>HMGIEY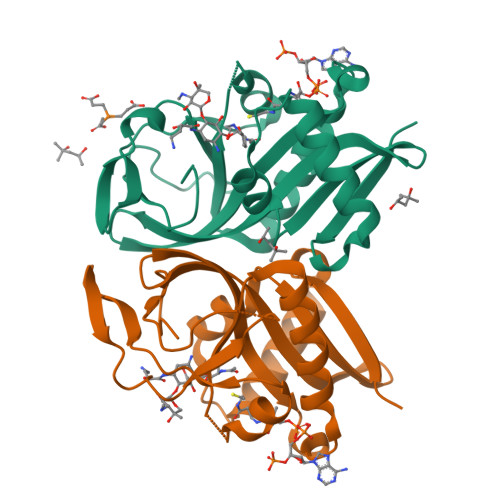RSLHTSQLTLSEKEALYDLLIEGFEGDFSHDDFAHTLGGMHVMAFDQQKLVGHVAIIQRHMALDNTPISVGYVEAMVVEQSYRRQGIGRQLMLQTNKIIASCYQLGLLSASDDGQKLYHSVGWQIWKGKLFELKQGSYIRSIEEEGGVMGWKADGEVDFTASLYCDFRGGDQW[2x]>MAVELGVLLVRPRPGTGLGRVMRTLLLVLWLATRGSALYFHIGETEKKCFIEEIPDETMVIGNYRTQLYDKQREEYQPATPGLGMFVEVKDPEDKVILARQYGSEGRFTFTSHTPGEHQICLHSNSTKFSLFAGGMLRVHLDIQVGEHANDYAEIAAKDKLSELQLRVRQLVEQVEQIQKEQNYQRWREERFRQTSESTNQRVLWWSILQTLILVAIGVWQMRHLKSFFEAKKLV[12x]

TMED9 is a member of the TMED family of cargo receptors that facilitate the bidirectional transport of membrane proteins at the endoplasmic reticulum (ER)–Golgi interface via anterograde COPII and retrograde COPI vesicles. In addition, all TMEDs share a conserved domain architecture with luminal Golgi-dynamics (GOLD) and coiled-coil (CC) domains and a single TM domain. Sorting signals for COPI (dilysine motif, KK) and COPII (diphenylalanine motif, FF) coatomer proteins are contained in the cytosolic tail of TMED9. Here, we report cryo–electron microscopy (cryo-EM) structures of full-length TMED9 in octameric and dodecameric forms.

An unexpected feature of the TMED9 oligomers is an intrinsic symmetry mismatch between the CC and TM domains. In the homo-dodecamer, the TM domain was formed by three tetramers, but the CC domain was formed by four trimers. In contrast to the symmetry of the TM domain, the CC domain formed obligate trimeric coiled coils, as was also predicted by MultiCoil. The experiment identified a number of PIPs, with PIP (36:2) containing two oleic acyl chains as the most prominent PIP species. PIP (36:2) fits well with the cryo-EM density at both the headgroup and the acyl chains. The location of the PIP molecules suggests that they may facilitate TM oligomerization. The PIP headgroup between the TM tetramers is within hydrogen bonding distance to the R223 and H224 side chains from two of the four subunits at the tetramer-tetramer interface; these interactions could further stabilize octameric, dodecameric, or higher-order TMED9 complexes. In addition, several hydrogen bonds may bridge the CC trimers to stabilize the oligomeric assemblies, such as those from E163, Q165, E173, Q177, K180, E181, N183, R186, R191, Q194, T195, Q201, R202, and W205. We have detected previously undescribed oligomeric forms of TMED9, including octameric, and dodecameric structures. These and, by extension, additional higher-order self-oligomerizing TMED9 structures, are stabilized by intrinsic symmetry mismatch between the TM and CC domains. Thus, not only can TMED9 oligomers recruit COPI but they may also exhibit enhanced interaction with COPI through increased avidity.>[2x]MNSNLPAENLTIAVNMTKTLPTAVTHGFNSTNDPPSMSITRLFPALLECFGIVLCGAIAG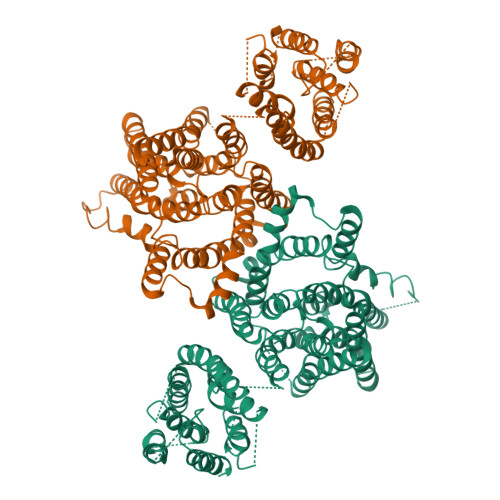AANVITSTQAKGLGNFVSRFALPALLFKNMVVLNFSNVDWSFLYSILIAKASVFFIVCVLTLLVASPDSRFSKAGLFPIFATQSNDFALGYPIVEALYQTTYPEYLQYIYLVAPISLMMLNPIGFIFCEIQKWKDTQNASQNKIKIVGLGLLRVLQNPIVFMVFIGIAFNFILDRKVPVYVENFLDGLGNSFSGSALFYLGLTMVGKIKRLKKSAFVVLILLITAKLLVLPLLCREMVELLDKGDSVVNHTSLSNYAFLYGVFPVAPGVAIFATQFNMEVEIITSGMVISTFVSAPIMYVSAWLLTFPTMDPKPLAYAIQNVSFDISIVSLISLIWSLAILLLSKKYKQLPHMLTTNLLIAQSIVCAGMMIWNFVKEKNFVGQILVFVLLYSSLYSTYLWTGLLAISLFLLKKRERVQIPVGIIIISGWGIPALLVGVLLITGKHNGDSIDSAFFYGKEQMITTAVTLFCSILIAGISLMCMNQTAQAGSYEGFDQSQSHKVVEPGNTAFEESPAPVNEPELFTSSIPETSCCSCSMGNGELHCPSIEPIANTSTSEPVIPSFEKNNHCVSRCNSQSCILAQEEEQYLQSGDQQLTRHVLLCLLLIIGLFANLSSCLWWLFNQEPGRLYVELQFFCAVFNFGQGFISFGIFGLDKHLIILPFKRRLEFLWNNKDTAENRDSPVSEEIKMTCQQFIHYHRDLCIRNIVKERRCGAKTSAGTFCGCDLVSWLIEVGLASDRGEAVIYGDRLVQGGVIQHITNEYEFRDEYLFYRFLQKSPEQSPPAINANTLQQERYKEIEHSSPPSHSPKTSRENLYFQ> MSIDSALNWDGEMTVTRFDSMTGAHFVIRLDSTQLGPAAGGTRAAQYSNLADALTDAGKLAGAMTLKMAVSNLPMGGGKSVIALPAPRHSIDPSTWARILRIHAENIDKLSGNYWTGPDVNTNSADMDTLNDTTEFVFGRSLERGGAGSSAFTTAVGVFEAMKATVAHRGLGSLDGLTVLVQGLGAVGGSLASLAAEAGAQLLVADTDTERVAHAVALGHTAVALEDVLSTPCDVFAPCAMGGVITTEVARTLDCSVVAGAANNVIADEAASDILH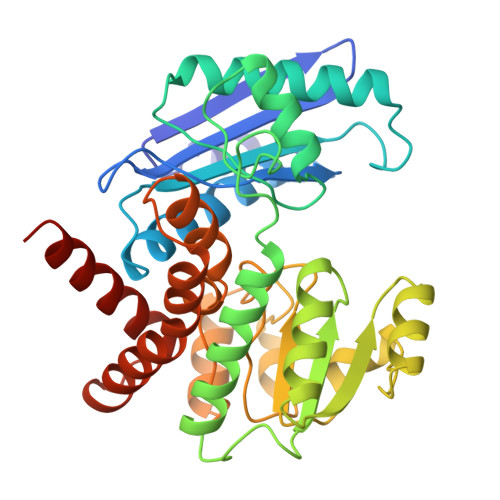ARGILYAPDFVANAGGAIHLVGREVLGWSESVVHERAVAIGDTLNQVFEISDNDGVTPDEAARTLAGRRAREASTTTATA>[2x]HHHHHHSSGLVPRGSHMTIFPDDFLWGGAVAANQVEGAYNEDGKGLSVQDVLPKGGLGEATENPTEDNLKLIGIDFYHKYKEDISLFSEMGFNVFRTSIAWSRIFPKGDEEEPNEAGLKYYDELFDELHAHGIEPLVTLSHYETPLYLARKYHGWVDRRMIHFYEKFARTVLERYKDKVKYWLTFNEVNSVLELPFTSGGIDIPKENLSKQELYQ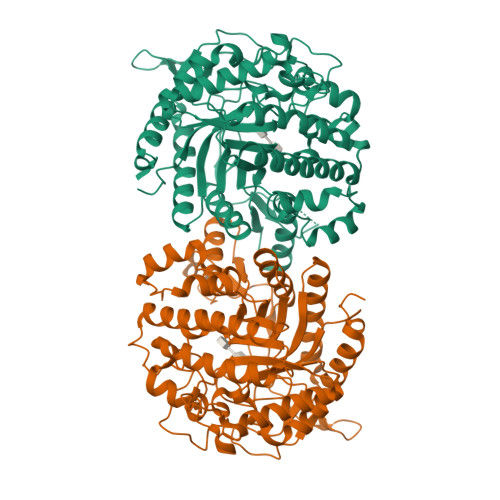AIHHELVASSLVTKIAREINSEFKVGCMVLAMPAYPMTPNPKDVWATHEYENLNYLFSDVHVRGYYPNYAKRYFKENDINIEFAAEDAELLKNYTVDFLSFSYYMSVTQSALPTQYNSGEGNIIGGLVNPYLESSEWGWQIDPIGLRIILNRYYDRYQIPLFIVENGLGAKDQLIKDELNNLTVQDDYRIQYMKEHLLQVAEALQDGVEIMGYTSWGCIDCVSMSTAQLSKRYGLIYVDRNDDGSGTLNRYKKMSFTWYKEVIESNGESLFK> MITTPLVHVASVEKGRSYEDFQKVYNAIALKLREDDEYDNYIGYGPVLVLLAWHISGTWDKHDNTGGSYGGTYRFKKEFNDPSNAGLQNGFKFLEPIHKEFPWISSGDLFSLGG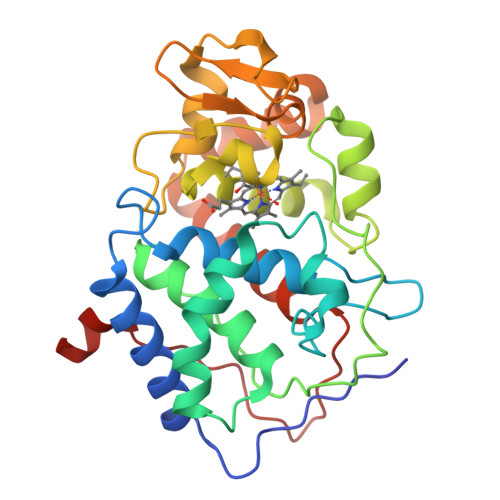VTAVQEMQGPKIPWRCGRVDTPEDTTPDNGRLPDADKDAGYVRTFFQRLNMNDREVVALMGAHALGKTHLKNSGYEGPWGAANNVFTNEFYLNLLNEDWKLEKNDANNEQWDSKSGYMMLPTDYSLIQDPKYLSIVKEYANDQDKFFKDFSKAFEKLLENGITFPKDAPSPFIFKTLEEQGL>[3x]DGANSDAAKEYLTKDSFSYEVYGIIAMQAAYRDYDSGD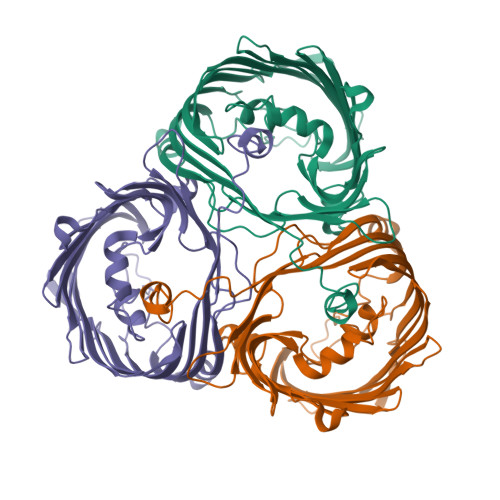AKQDDNLGGMQLNNESRIGFRGKKQFANFEPTFIWQIEGGYVDPSFGGEGAGLGERDTFVGFESASWGQVRLGRVLTPMYELVDWPASNPGLGDVYDWGGAIGGAKYQDRQSNTIRWDSPMYADKFSIDAAVGAGDKAGLGAGDDYWGGIAAHYKLGPLQLDAAYEGNRNIEAEGQTWENNTYLVGVQGWFENGISFFAQYKYMEADASNGVNEKQDAMSAGLMYTTGDWQYKLGYAANFDLERDGKTLSNTSDDVVSAQIMYFVDPSAVLYARARMNDFNEGLDGLDDAARWTSGTNGDYNEYSVGVEYYF> MAFHEVRFPANLSFGSVGGPERRTEIVTLSSGHEERNSPWAHSRRHYDAGVGLRSLDDVERLIAFFEARGGQLHGFRWKDWADFKSCPASRAVAHEDQLIGMGDGVTTAFQLVKTYVSGGQSYLRPIVKPVEGTVKLGIAGDHQAEAVNFA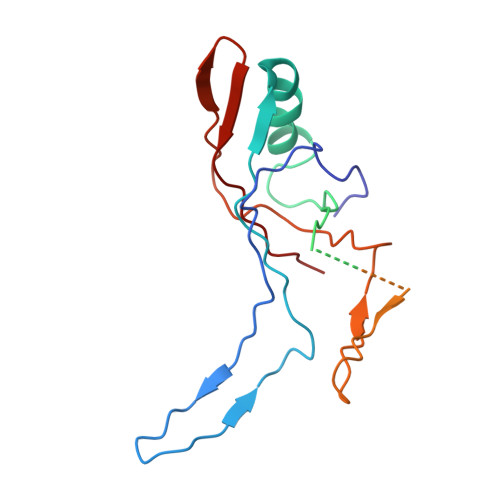VDHATGIVSFNEPPPQGARVTAGFEFDVPVRFDTDRIAVSVQSFQAGDLPQVPVVEVRI> MAPLRKTAVLKLYVAGNTPNSVRALKTLNNILEKEF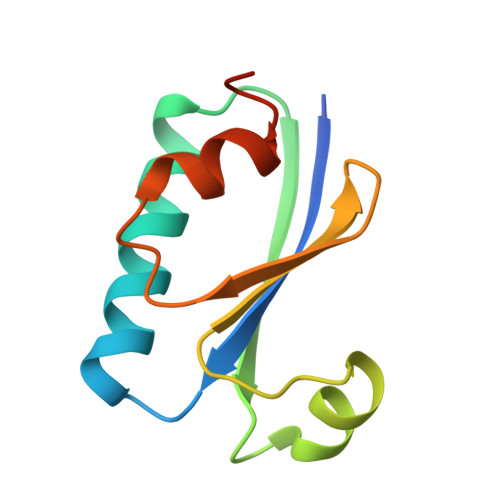KGVYALKVIDVLKNPQLAEEDKILATPTLAKVLPPPVRRIIGDLSNREKVLIALRLLAEEIGD>[8x]MTEAQAIAKQLGGVKPDDEWLQAEIARLKGKSIVPLQQVKTLHDWLDGKRKARKSCRVVGESRTGKTVACDAYRYRHKPQQEAGRPPTVPVVYIRPHQKCGP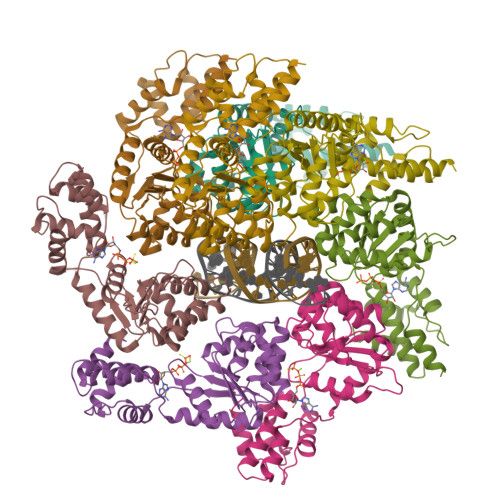KDLFKKITEYLKYRVTKGTVSDFRDRTIEVLKGCGVEMLIIDEADRLKPETFADVRDIAEDLGIAVVLVGTDRLDAVIKRDEQVLERFRAHLRFGKLSGEDFKNTVEMWEQMVLKLPVSSNLKSKEMLRILTSATEGYIGRLDEILREAAIRSLSRGLKKIDKAVLQEVAKEYK> MNNMNVIIADDHPIVLFGIRKSLEQIEWVNVVGEFEDSTALINNLPKLDAHVLITDLSMPGDKYGDGITLIKYIKRHFPSLSIIVLTMNNNPAILSAVLDLDIEGIVLKQGAPTDLPKALAALQKGKKFTPESVSRLLE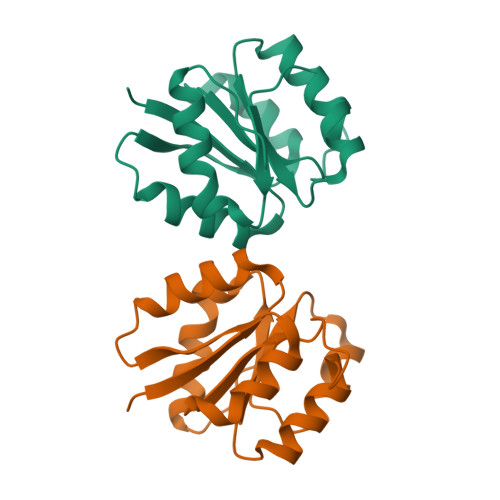KISAGGYG> PKRELEQGVAFSDLCNFLVTPTVQGWKVYWAGLEFDVNQKGITLLNRLKVNDFAPAWAMTRNLFPHLFKNQQSEVQTPIWALRVILAAGILDQLMDHSLIEPLSGALNLIADWLLTTSTNHFNMRTQRVKDQLSMRMLSLIRSNIINFINKLETLHVVNYKGLLSSVEIGTPSYAIIITRTNMGYLVEVQEPDKSAMDIRHPGPVKFSLLHESTLK

VP24, one of only eight proteins encoded by ebolaviruses, functions in virus replication and assembly, and is thought to contribute to immune suppression by binding to a certain class of molecules called karyopherins to prevent them from transporting a transcription factor termed STAT1. In addition to its role in interferon antagonism, ebolavirus VP24 has also been proposed to associate with membranes, and is important for assembly and function of the viral ribonucleoprotein complex (RNP), where VP24 binds to the viral nucleoprotein NP. VP24 adopts a compact, single domain, α/β structure of novel fold (DaliLite v.3). The overall shape of VP24 resembles a triangular pyramid of dimensions 73 Å×30 Å×30 Å.

In order to provide 3D templates for understanding VP24 and its many roles in immune evasion, replication and assembly, we crystallized VP24 from Sudan virus (two versions crystallized: SUDV1–233 and SUDV11–233) and Reston virus (one version crystallized: RESTV11–237). We determined the structure of SUDV11–233 at 2.1 Å resolution by multiwavelength anomalous diffraction (MAD) using selenomethionine-incorporated protein expressed recombinantly in E. coli. Crystal structures presented here include VP24 from an ebolavirus that is pathogenic to humans (Sudan virus; SUDV) and VP24 from an ebolavirus that thus far, appears nonpathogenic to humans (Reston virus; RESTV), although it is lethal to nonhuman primates. The overall folds of SUDV and RESTV VP24 are similar, as expected (r.m.s.d. of 0.81 Å; also see Figure S2b for structural alignment). The entrance to the hydrophobic cavity (11 Å wide) appears to be gated by two residues (Y172 and M71) that point away from each other in RESTV VP24 but toward each other in SUDV VP24, appearing to block the hydrophobic cavity. Crystal packing can sometimes illustrate biologically relevant assemblies, but no tetrameric or other higher oligomeric interactions are observed in crystals of SUDV or RESTV VP24. One pairwise VP24-VP24 interaction is conserved in the crystal packing between the SUDV (P3121) and RESTV VP24 (P1211) structures, although it is currently unclear if it is biologically relevant. This interaction involves α1, β1–3 and the N-terminal region of α8, and buries residue L147 that was previously implicated for virulence, although 142–146 remain solvent exposed. Another crystal lattice interaction observed in both RESTV and SUDV structures involves packing of the hydrophobic N-terminal regions of VP24 into the Face 3 pocket of a neighboring molecule.>SAHTESVCVHAGTATGADLHWLNAICTGKSTYTVNCAPAGNKNAGSTHTGTCPAGQDCFQLEQVGNFWGDREPDATCSPSNTVFDAVDDKEATHVNGKVVTRAGKPGIGRKLIRLKAQVYRRDGHYGQTSRMGFFRNGKEVYHIDNVASMEPTWNFDPSSDQSFSFFFTPGPNAFRIQGTLNLAS[2x];>[2x]GPMLPKGEEGDIIGTFNFSSSDSQPLK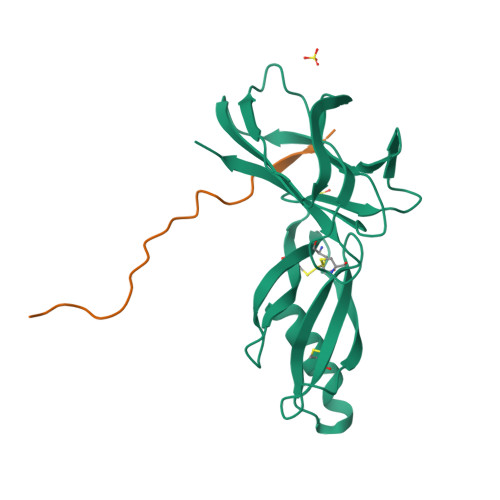IHWVDTPDSSGSNLVPR> SITSSLGYPTLRIEKNDLRSVTLLEAKGKVKDIAISRERITLKDVLQEGTFGRIFHGILIDEKDPNKEKQAFVKTVKDQASEIQVTMMLTESCKLRGLHHRNLLPITHVCIEEGEKPMVILPYMNWGNLKLFLRQCKLVEANNPQAISQQDLVHMAIQIACGMSYLARREVIHKDLAARNCVIDDTLQVKITDNALSRDLFPMDYHCLGDNENRPV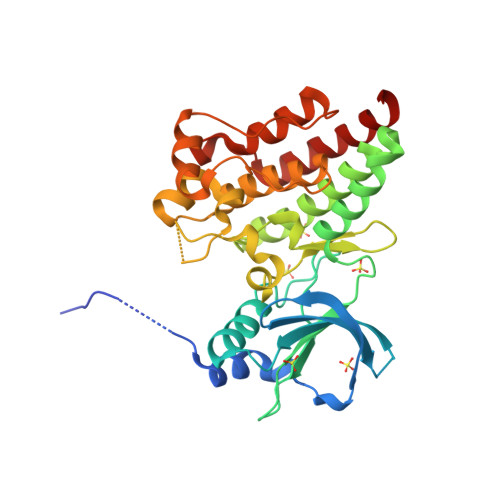RWMALESLVNNEFSSASDVWAFGVTLWELMTLGQTPYVDIDPFEMAAYLKDGYRIAQPINCPDELFAVMACCWALDPEERPKFQQLVQCLTEFHAALGAYV> GPLGSGRPKQQLLRAATGKAILNGIDSINKVLDH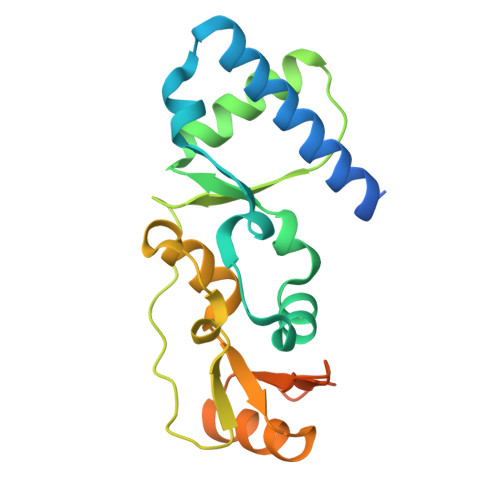FRRKGINQHVQNGYHGIVMNNFECEPAFYTCVEVTAGNRLFYHIVDSDEVSTKILMEFNKMNLPGEVTFLPLNKLDVRDTAYPETNDAIPMISKLRYNPRFDKAFKHVFGKTLICRSMEVSTQLARAFTMDCITLEGDQVSHRGALTGGYYDTRKSRLELQKDVRKA Deoxynivalenol (DON) is a toxicologically relevant trichothecene mycotoxin frequently found in cereal products. GSH-mediated epoxide opening and Michael addition are typical reactions catalyzed by glutathione transferases (GSTs, EC 2.5.1.18) and investigating the capacity of GSTs to detoxify DON appears to be promising. The serine-type classes tau (GSTU) and phi (GSTF) are prevalent in plants and are crucial for herbicide resistance of crop plants. Investigation of the transcriptome of F. graminearum–infected wheat allowed us to identify pathogen-inducible tau class GSTs capable of catalyzing DON-10-GSH and/or DON-13-GSH formation.

TaGST-10 was cocrystallized with its reaction product, DON-13-GSH, to observe substrate/product binding at the active site. TaGST-10 crystallized as a dimer in the asymmetric unit and contained a molecule of DON-13-GSH in each active site. Similar to S-hexyl-GSH in TaGSTU4, the GSH moiety of DON-13-GSH is mainly bound by polar interactions involving hydrogen bonds between Glu70 and Ser71 with the glutamyl residue, Val58 with the cysteinyl residue, and Lys44 with the glycine residue of GSH. The catalytic serine of TaGST-10 forms a hydrogen bond with the cysteinyl-sulfur of DON-13-GSH. The DON moiety of DON-13-GSH is in close proximity to the hydrophobic residues Val12, Pro18, Trp173, and Phe220. The only polar interaction with DON is a hydrogen bond between the hydroxy group of Ser116 with the C15 oxygen of DON. Replacing Ser116 by Val resulted in clearly reduced DON-13-GSH synthesis by TaGST-10 S116V. This implies that Ser116 contributes to DON binding in an orientation favoring nucleophilic attack of GSH at the C13 position of DON. DON-13-cysteine is located at the entrance of a cavity located between the two domains of chain A. This cavity is formed by residues on α1, β2, and the loop connecting α8 and α9.

>[2x]GHMAGGGSDEVKLLGMWASPFVLRVQLALSLKGVGYEYVEEDLKSKSELLLKSNPVLQKVPVLIHDGKPVCESSVILQYIDEAFAGVGPSLLPEEPHGRAVARFWAAYIDGTLVKASSQASMAKTEEEKAEGKKQVTAAVETLEGALRDCSNGKPFFGGDTAGYVDVMLGGLLAWVHAGDKMKGVKTFDPATTPLLAAWADNFGSLDAVEAVMPDVGKLVEFAMAMHARAAAAATN> 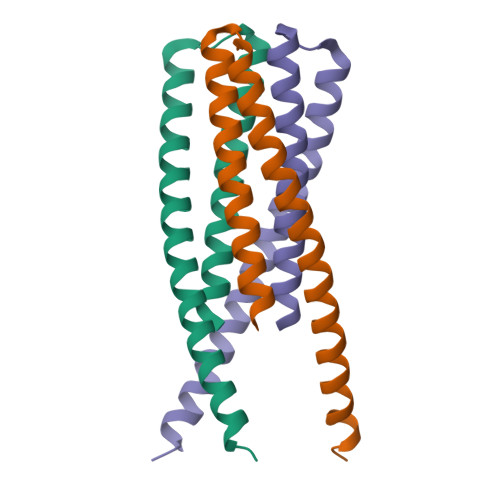MASMTGGQQMGRGSGIVQQQSNLLRAIEAQQHLLQLTVWGIKQGGGGSEWEREISNYTDIIYRLIEESQNQQEKNEQELLALDKWASLWNWFDITNWLWYIQHHHHHH6-deoxy-beta-L-fructofuranose | C6 H12 O5 | 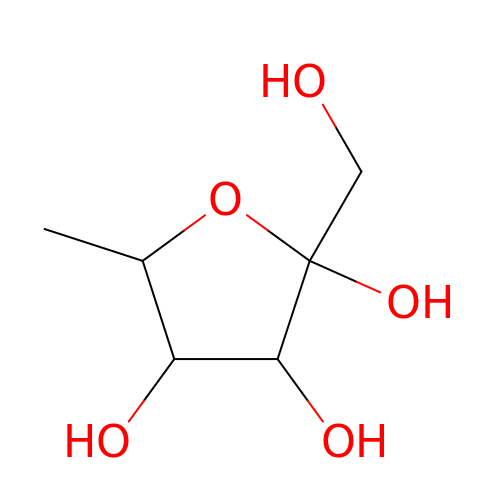CJJCPDZKQKUXSS-AZGQCCRYSA-N> SMENKNLNYILGLDLGIASVGWAVVEIDEKENPLRLIDVGVRTFERAEVPKTGESLALSRRLARSARRLTQRRVARLKKAKRLLKSENILLSTDERLPHQVWQLRVEGLDHKLERQEWAAVLLHLIKHRGYLSQRKNESKSENKELGALLSGVDNNHKLLQQATYRSPAELAVKKFEVEEGHIRNQQGAYTHTFSRLDLLAEMELLFSRQQHFGNPFASEKLLENLTALLMWQKPALSGEAILKMLGKCTFEDEYKAAKNTYSAERFVWITKLNNL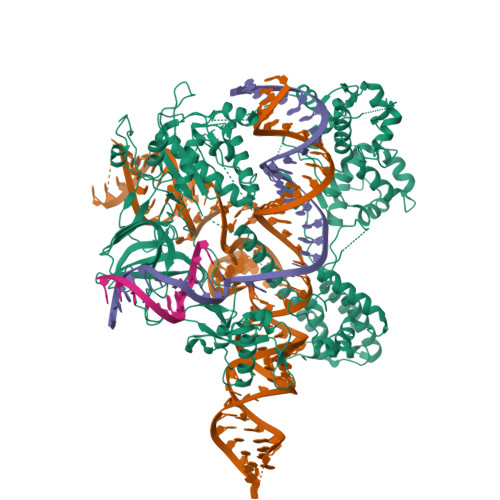RIQENGLERALNDNERLALMEQPYDKNRLFYSQVRSILKLSDEAIFKGLRYSGEDKKAIETKAVLMEMKAYHQIRKVLEGNNLKAEWAELKANPTLLDEIGTAFSLYKTDEDISAYLAGKLSQPVLNALLENLSFDKFIQLSLKALYKLLPLMQQGLRYDEACREIYGDHYGKKTEENHHFLPQIPADEIRNPVVLRTLTQARKVINGVVRLYGSPARIHIETGREVGKSYKDRRELEKRQEENRKQRENAIKEFKEYFPHFAGEPKAKDILKMRLYKQQNAKCLYSGKPIELHRLLEKGYVEVDAALPFSRTWDDSFNNKVLVLANENQNKGNLTPFEWLDGKHNSERWRAFKALVETSAFPYAKKQRILSQKLDEKGFIERNLNDTRYVARFLCNFIADNMHLTGEGKRKVFASNGQITALLRSRWGLAKSREDNDRHHALDAVVVACSTVAMQQKITRFVRFEAGDVFTGERIDRETGEIIPLHFPTPWQFFKQEVEIRIFSDNPKLELENRLPDRPQANHEFVQPLFVSRMPTRKMTGQGHMETVKSAKRLNEGISVIKMPLTKLKLKDLELMVNREREKDLYDTLKARLEAFNDDPAKAFAEPFIKKGGAIVKSVRVEQIQKSGVLVREGNGVADNASMVRVDVFTKGGKYFLVPIYTWQVAKGILPNKAATQYKDEEDWEVMDNSATFKFSLHPNDLVKLVTKKKTILGYFNGLNRATGNIDIKEHDLDKSKGKQGIFEGVGIKLALSFEKYQVDELGKNIRLCKPSKRQPVR> MIKATDRKLVVGLEIGTAKVAALVGEVLPDGMVNIIGVGSCPSRGMDKGGVNDLESVVKCVQRAIDQAELMADCQISSVYLALSGKHISCQNEIGMVPISEEEVTQEDVENVVHTAKSVRVRDEHRVLHVIPQEYAIDYQEGIKNPVGLSGVRMQAKVHLITCHNDMAKNIVKAVERCGLKVDQLIFAGLASSYSVLTEDERELGVCVVDIGGGTMDIAVYTGGALRHTKVIPYAGNVVTSDIAYAFGTPPSDAEAIKVRHGCALGSIVGKDESVEVPSVGGRPPRSLQRQTLAEVIEPRYTELLNLVNEEILQLQEKLRQQGVKHHLAAGIVLTGGAAQIEG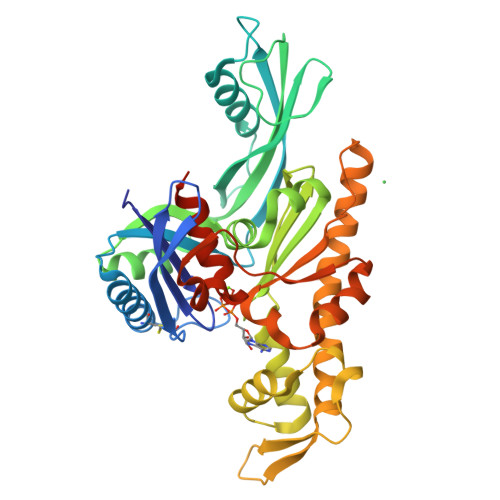LAACAQRVFHTQVRIGAPLNITGLTDYAQEPYYSTAVGLLHYGKESHLNGEAEVEKRVTASV>TRDQNGTWEMESNENFEGYMKALDIDFCTRKIAVRCTQTKVIDQDGDNFKDKTTSTHRNY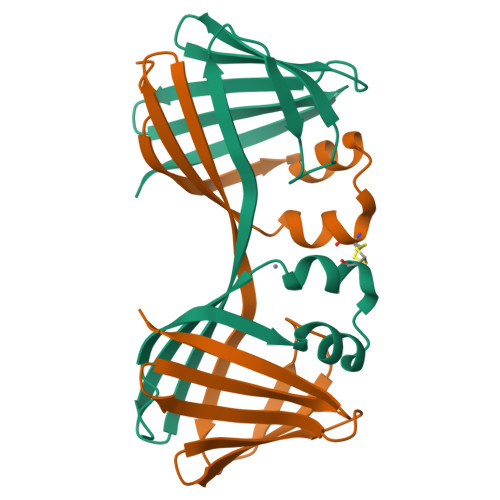DVDFTVGVEFDEYTKSLDNRHVKALVTWEGDVLVCVQKGEKENRGWKKWIEGDKLYLELTCGDQVCRQVFKKK[2x]> MQQLNENKIIKLLRDNIPKLQLIYLFGSYSQGTQHRNSDIDIAVLAADTLDNIARWELAQKLASALDSDVDLVDLRSASTVLCQQVVTQGKQLWGTQQDDELFAVKTISMYQHLQAERQAIIDDVMANTAAKAHRGESL;>MNDIIINKIATIKRCIKRIQQVYGDGSQFKQDFTLQDSVILNLQRCCEACIDIANHINRQQQLGIPQSSRDSFTLLAQNNLITQPLSDNLKKMVGLRNIAVHDYQELNLDIVVHVVQHHLEDFEQFIDVIKAEHHHHH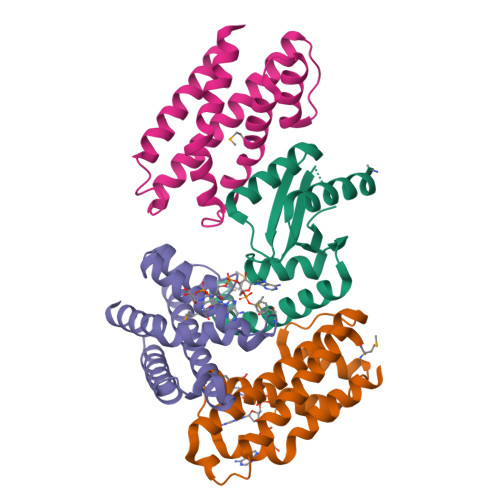H[3x]> DLSASVPTRPAEPERKTLADYGGYPSALDAVKQKNDAAVAAYLENAGDSAMAENVRNEWLKSLGARRQWTLFAQEYAKLEPAGRAQEVECYADSSRNDYTRAAELVKNTGKLPSGCTKLLEQAAASGLLDGNDAWRRVRGLLAGRQTTDARNLAAALGSPFDGGTQGSREYALLNVIGKEARKSPNAAALLSEMESGLSLEQRSFAWGVLGHYQSQNLNVPAALDYYGKVADRRQLTDDQIEWYARAALRARRWDELASVISHMPEKLQKSPTWLYWLARSRAATGNTQEAEKLYKQAAATGRNFYAVLAGEELGRKIDTRNNVPDAGKNSVRRMAEDGAVKRALVLFQNSQSAGDAKMRRQAQAEWRFATRGFDEDKLLTAAQTAFDHGFYDMAVNSAERTDRKLNYTLRYISPFKDTVIRHAQNVNVDPAWVYGLIRQESRFVIGAQSRVGAQGLMQVMPATAREIAGKIGMDAAQLYTADGNIRMGTWYMADTKRRLQNNEVLATAGYNAGPGRARRWQADTPLEGAVYAETIPFSETRDYVKKVMANAAYYAALFGAPHIPLKQRMGIVPAR

LtgA is responsible for the release of cytotoxic PG monomers from Neisseria pathogenic species. LtgA shares approximately 33% similarity in the C-terminal domain to its soluble periplasmic E. coli counterpart, Slt70, but is predicted to be an outer-membrane lipoprotein that is localized to the septum of N. gonorrhoeae. LtgA is a “heart-shaped” highly alpha-superhelical structure consisting of 37 α-helices. LtgA has three distinct domains: the C-domain, which is the catalytic domain, and the L and U-domains for which the function is unknown.

To evaluate the potential of bulgecin A as a broad-spectrum inhibitor for Lts, we solved the high-resolution crystal structures of the membrane bound Lt (LtgA) from the Neisseria species in complex with bulgecin A. The near atomic resolution structure of the LtgA-bulgecin A complex shows the complete structure of bulgecin A supported by a well-defined solvent model that clearly shows highly conserved residues interacting directly with bulgecin A and those that are engaged via water mediated interactions. Bulgecin A consists of a 4-O-sulfonyl-N-acetylglucosamine moiety that is linked by a β 1-4 glycosidic linkage to a 4-hydroxy-5-(hydroxymethyl)-l-proline that terminates with a taurine (N-linked sulfur) moiety. Bulgecin A is bound in the region of the active site defined as subsite −1, −2, −3, and partially occludes subsite +1. In the active site of LtgA, chitopentaose and bulgecin A have overlapping binding sites. This strongly suggests that bulgecin A could be competitive with the PG glycan strand. In subsite −2, the GlcNAc residue forms direct hydrogen bonds with the side chains of Y532 and T504 and with the main chain of M501 and Y551. In subsite −1, the hydroxyl-methyl of the proline is directly hydrogen bonded to the OE2 of the catalytic residue E481 and the ND2 of N552. The taurine group of the inhibitor is directly hydrogen bonded to S490 and E580. The OS1 and OS2 of the sulphonated portion of the taurine is directly hydrogen bonded to the main chain and side chain of R491. Bulgecin A appears to mimic the oxocarbonium intermediate step in the predicted mechanism of Lts and is most likely competitive with the glycan strand of the PG.>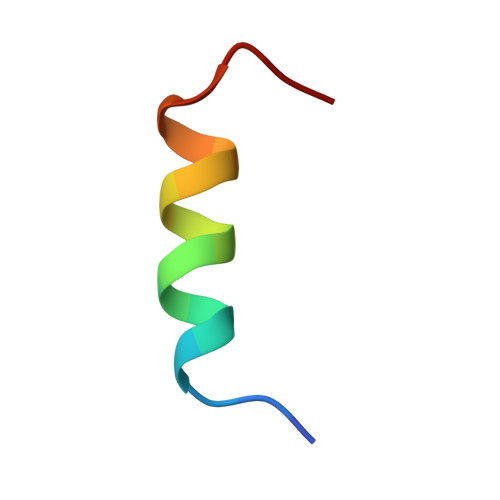 LSEGLRESLSSYISLAEDP> IAGGEAIYAAGGGRCSLGFNVRSSSGATYALTAGHCTEIASTWYTNSGQTSLLGTRAGTSFPGNDYGLIRHSNASAADGRVYLYNGSYRDITGAGNAYVGQTVQRSGSTTGLHSGRVTGLNATVNYGGGDIVSGLIQTNVCAEPGDSGGALFAGSTALGLTSGGSGNCRTGGTTFFQ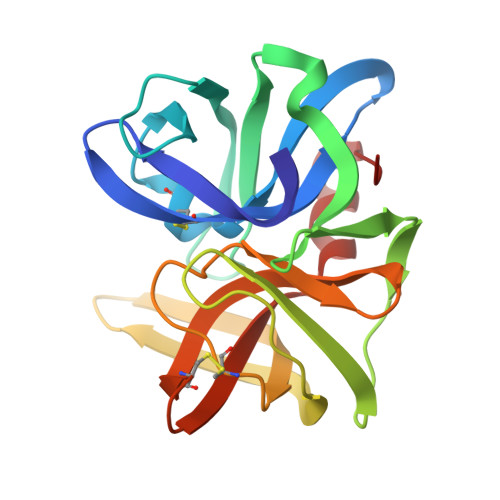PVTEALSAYGVSIL>[4x]MYEPKPEHRFTFGLWTVGNVGRDPFGDAVRERLDPVYVGHKLAELGVHGVNLHDEDLIPRGTPPQERDQIVRRFKRALDETGLKVPMVTGNLFSDPGFKDGGFTSRDPWVRAYAFRKSLETMDLGAELGAEIYVVWPGREGAEVEATGKARKVWDWVR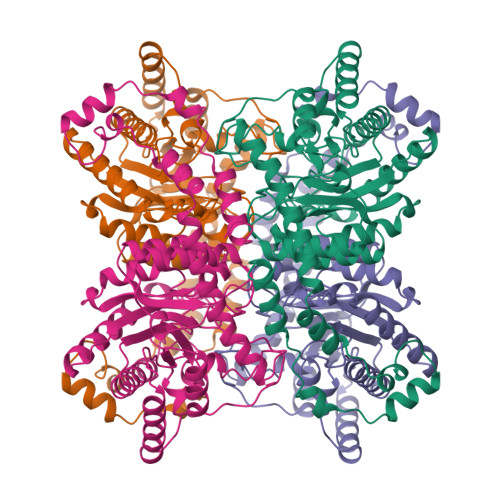EPLNFMAAYAEDQGYGYRFALEPKPNEPRGDIYFATVGSMLALIHTLERPERFGLNPEFAHETMAGLNFVHAVAQALDAGKLLHIDLNGQRMNRFDQDLRFGSENLKAAFLLVDLLESSGYQGPRHFDAHALRTEDEEGVWAFARGCMRTYLILKERAEAFREDPEVKELLAAYYQEDPAALPLMDPYSHEKAEALKRAELPLEAKRHRGYALERLDQLAVEYLLGVRG Enterovirus 70 (EV70) is a human pathogen belonging to the family Picornaviridae. EV70 is transmitted by eye secretions and causes acute hemorrhagic conjunctivitis, a serious eye disease. The capsid of EV70 is composed of the subunits VP1, VP2, VP3, and VP4. The major capsid proteins of EV70 are organized with pseudo-T=3 icosahedral symmetry, with VP1 subunits forming pentamers around 5-fold symmetry axes and VP2 and VP3 subunits forming heterohexamers at 3-fold axes of the capsid.

The structures of altered and empty particles of EV70 were determined to resolutions of 3.7 and 4.3 Å, respectively. The altered particle lacks VP4 subunits and is expanded 4% in diameter compared to the native virion. The expansion is enabled by the loosening of contacts between the pentamers of capsid protein protomers, which is accompanied by a reduction in the interpentamer binding interface from 3,350 to 2,750 Å2. The first 48 N-terminal residues and loops BC (residues 84 to 91) and DE (residues 134 to 142) of VP1, loop AB (residues 43 to 57) of VP2, and loops BC (residues 73 to 78) and GH (residues 170 to 172) of VP3 are not resolved in the cryo-EM reconstruction of the altered particle. Amino acid residues 49 to 56 from the N terminus of VP1 cross the capsid of the altered particle of EV70, resulting in the exposure of the N terminus of VP1 at the surface of the altered particle. The N termini of the VP1 subunits pass through the capsid approximately between a 2-fold axis of the altered particle and the canyon. The externalization of the N terminus of VP1 is enabled by a conformational change and a shift of the GH loop of VP3 away from an interprotomer interaction interface. The pocket inside the VP1 subunit in the altered particle of EV70 is collapsed, as is also the case in altered particles of other enteroviruses that were characterized previously. The collapse of the pocket of EV70 is enabled by the movement of VP1 strands B, C, H, and I into the pocket. The altered particle of EV70 contains approximately rectangular pores of 17 by 4 Å positioned on 2-fold symmetry axes of the capsid.

> ATTQIGEIVKTVANTVESEIKAELGVIPSLNAVETGATSNTEPEEAIQTRTVINMHGTAECLVENFLGRSALVCMRSFEYKNHSTSTSSIQKNFFIWTLNTRELVQIRRKMELFTYLRFDTEITIVPTLRLFSSSNVSFSGLPNLTLQAMYVPTGARKPSSQDSFEWQSACNPSVFFKINDPPARLTIPFMSINSAYANFYDGFAGFEKKATVLYGINPANTMGNLCLRVVNSYQPVQYTLTVRVYMKPKHIKAWAPRAPRTMPYTNILNNNYAGRSAAPNAPTAIVSHRSTIKTMPNDINLTTA;> SPSAEACGYSDRVLQLKLGNSSIVTQEAANICCAYGEWPTYLPDNEAVAIDKPTQPETSTDRFYTLKSKKWESNSTGWWWKLPDALNQIGMFGQNVQYHYLYRSGFLCHVQCNATKFHQGTLLIVAIPEHQIGKKGTGTSASFAEVMKGAEGGVFEQPYLLDDGTSLACALVYPHQWINLRTNNSATIVLPWMNSAPMDFALRHNNWTLAVIPVCPLAGGTGNTNTYVPITISIAPMCAEYNGLRNAITQ;> GVPTCLLPGSNQFLTTDDHSSAPAFPDFSPTPEMHIPGQVHSMLEIVQIESMMEINNVNDASGVERLRVQISAQSDMDQLLFNIPLDIQLEGPLRNTLLGNISRYYTHWSGSLEMTFMFCGSFMTTGKLIICYTPPGGSSPTDRMQAMLATHVVWDFGLQSSITIIIPWISGSHYRMFNTDAKAINANVGYVTCFMQTNLVAPVGAADQCYIVGMVAAKKDFNLRLMRDSPDIGQSAILPEQ>[2x]MPPLSLLIKPASSGCNLKCTYCFYHSLSDNRNVKSYGIMRDEVLESMVKRVLNEANGHCSFAFQGGEPTLAGLEFFEKLMELQRKHNYKNLKIYNSLQTNGTLIDESWAKFLSENKFLVGLSMDGPKEIHNLNRKDCCGLDTFSKVE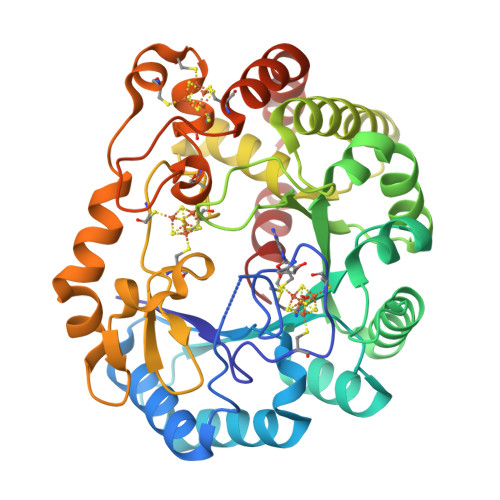RAAELFKKYKVEFNILCVVTSNTARHVNKVYKYFKEKDFKFLQFINCLDPLYEEKGKYNYSLKPKDYTKFLKNLFDFWYEDFLNGNRVSIRYFDGLLETILLGKSSSCGMNGTCTCQFVVESDGSVYPCDFYVLDKWRLGNIQDMTMKELFETNKNHEFIKLSFKVHEECKKCKWFRLCKGGCRRCRDSKEDSALELNYYCQSYKEFFEYAFPRLINVANNIKSDPNSSSVDKLAAALEHHHHHH> 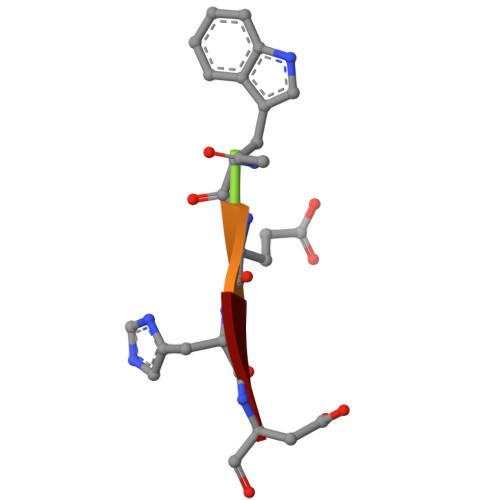XWEHD>[2x]GKKVLIVYAHQEPKSFNGSLKNVAVD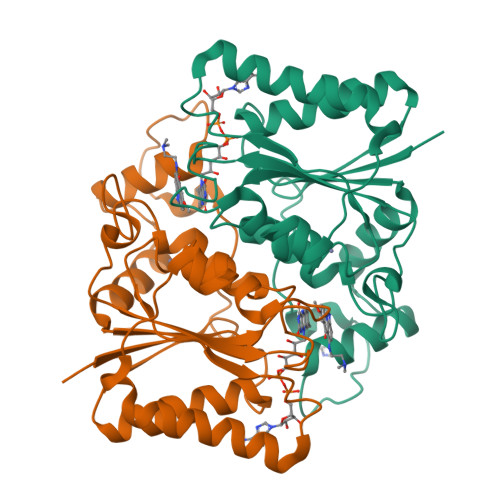ELSRQGCTVTVSDLYAMNFEPRATDKDITGTLSNPEVFNYGVETHEAYKQRSLASDITDEQKKVREADLVIFQFPLYWFSVPAILKGWMDRVLCQGFAFDIPGFYDSGLLQGKLALLSVTTGGTAEMYTKTGVNGDSRYFLWPLQHGTLHFCGFKVLAPQISFAPEIASEEERKGMVAAWSQRLQTIWKEEPIPCTAHWHFG>[8x]MTEGLFPRGRKVRVVSTLGPASSTAEQIRDRFLAGADVFRINMSHGTHDEKKVIVDNIRALEKEFNRPTTILFDLQGPKLRVGDFKEGKVQLKEGQTFTFDQDPTLGDETRVNLPHPEIFKALDKGHRLLLDDGKIVVRCVESSPTKIVTRVEVPGPLSDHKGFNVPDVVIPLAALTPKDRKDLDFALKEKADWVALSFVQRVE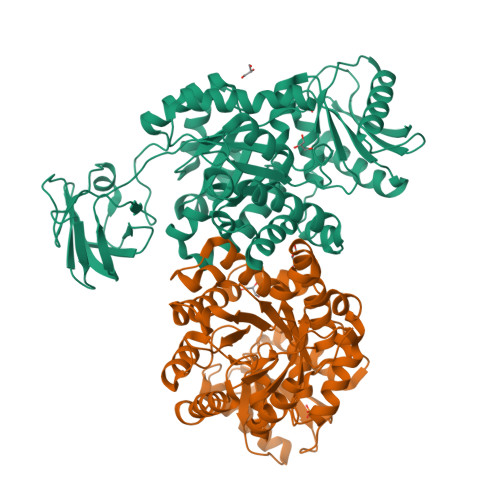DVIEAKELIKGRAPLLVKLEKPAAIENLESILAATDAVMVARGDLGVECLPESVPPTQKRIVERSRQLGKPVVVATAMLESMIKAPAPTRAEVSDVANAIYEGADGIMLSAESAAGDWPHEAVNMMHRIASYVENAPGYIERVRFTPTPAEPTTVDALAENASKTAETVGAKAIIVFTETGKTAQRVSRARPVAPILSLTPDAEVARRLGLVWGAQPVQVSTVKTLDEAKKLAAETAKKYGFAKAGDKLVVVAGEPFGKAGTTNIVDVIEA>AMADTIVAVELDSYPNTDIGDPNYPHIGIDIKSIRSKSTARWNMQTGKVGTVHISYNSVAKRLSAVVSYSGSSSTTVSYDVDLNNVLPEWVRVGLSATTGLYKETNTILSWSFTSKLKTNSIADANSLHFSFNQFSQNPKDLILQGDAFTDSDGNLQLTKVSSSGDPQGNSVGRALFYAPVHIWEKSAVVASFDATFTFLIK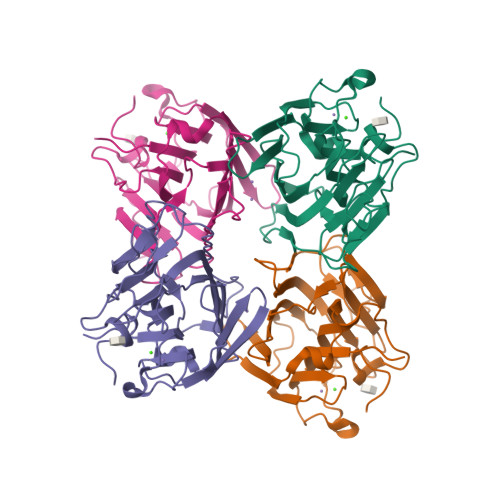SPDREPADGITFFIANTDTSIPSGSGGRLLGLFPDAN[4x]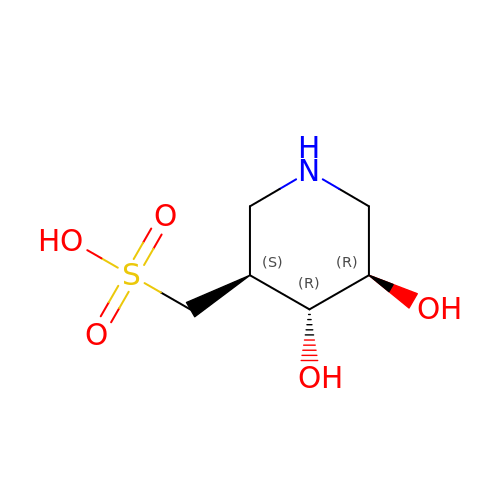[(3~{S},4~{R},5~{R})-4,5-bis(oxidanyl)piperidin-3-yl]methanesulfonic acid | C6 H13 N O5 S | RCSXCFCCYYFFCY-HSUXUTPPSA-N>[2x]GSHMKDLRSPICCILGHVDTGKTKLLDKIRQTNVQGGEAGGITQQIGATYFPIDAIKAKTKVMAEYEKQTFDVPGLLVIDTPGHESFSNLRSRGSSLCNIAILVIDIMHGLEQQTIESIKLLRDRKAPFVVALNKIDRLYDWKAIPNNSFRDSFAKQSRAVQEEFQSRYSKIQLELAEQGLNSELYFQNKNMSKYVSIVPTSAVTGEGVPDLLWLLLELTQKRMSKQLMYLSHVEATILEVKVVEGFGTTIDVILSNGYLREGDRIVLCGMNGPIVTNIRALLTPQPLRELRLKSEYVHHKEVKAALGVKIAANDLEKAVSGSRLLVVGPEDDEDELMDDVMDDLTGLLDSVDTTGKGVVVQASTLGSLEALLDFLKDMKIPVMSIGLGPVYKRDVMKASTMLEKAPEYAVMLCFDVKVDKEAEQYAEQEGIKIFNADVIYHLFDSFTAYQEKLLEERRKDFLDYAIFPCVLQTLQII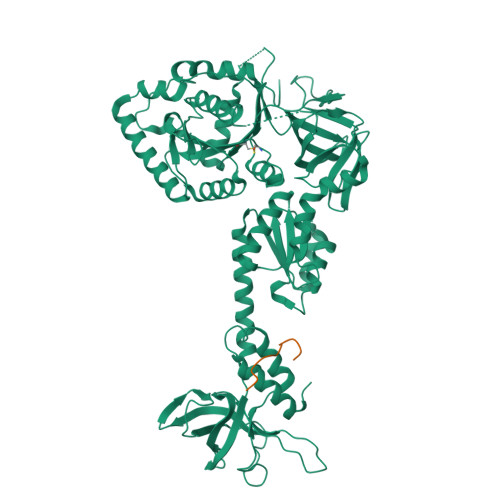NKRGPMIIGVDVLEGTLRVGTPICAVKTDPTTKERQTLILGKVISLEINHQPVQEVKKGQTAAGVAVRLEDPSGQQPIWGRHVDENDTLYSLVSRRSIDTLKDKAFRDQVARSDWLLLKKLKVVFGIE;> GSHMIYKEEGQEYAQITKMLGNGRVEASCFDGNKRMAHIRGKLRKKVWMGQGDIILVSLRDFQDDQCDVVHKYNLDEARTLKNQGELPENAKINETDNFGFESDEDVNFEFGNADEDDEEGEDEELDIDDI> QYSPNTQQGRTSIVHLFEWRWVDIA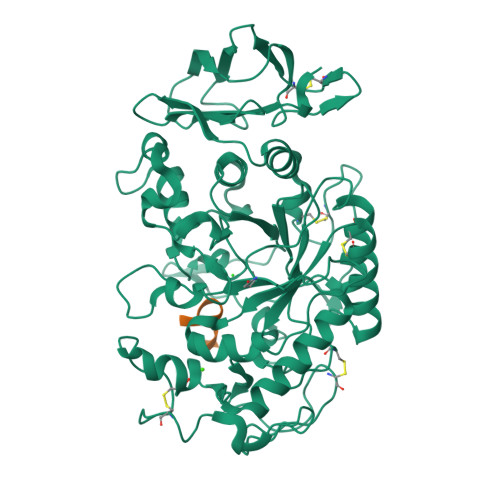LECERYLAPKGFGGVQVSPPNENVAIYNPFRPWWERYQPVSYKLCTRSGNEDEFRNMVTRCNNVGVRIYVDAVINHMCGNAVSAGTSSTCGSYFNPGSRDFPAVPYSGWDFNDGKCKTGSGDIENYNDATQVRDCRLTGLLDLALEKDYVRSKIAEYMNHLIDIGVAGFRLDASKHMWPGDIKAILDKLHNLNSNWFPAGSKPFIYQEVIDLGGEPIKSSDYFGNGRVTEFKYGAKLGTVIRKWNGEKMSYLKNWGEGWGFVPSDRALVFVDNHDNQRGHGAGGASILTFWDARLYKMAVGFMLAHPYGFTRVMSSYRWPRQFQNGNDVNDWVGPPNNNGVIKEVTINPDTTCGNDWVCEHRWRQIRNMVIFRNVVDGQPFTNWYDNGSNQVAFGRGNRGFIVFNNDDWSFSLTLQTGLPAGTYCDVISGDKINGNCTGIKIYVSDDGKAHFSISNSAEDPFIAIHAESKL;> XYPYSCWVRHX>[2x]GAMGRRLGVMGGTFDPIHYGHLVAASEVADLFDLDEVVFVPSGQPWQKGR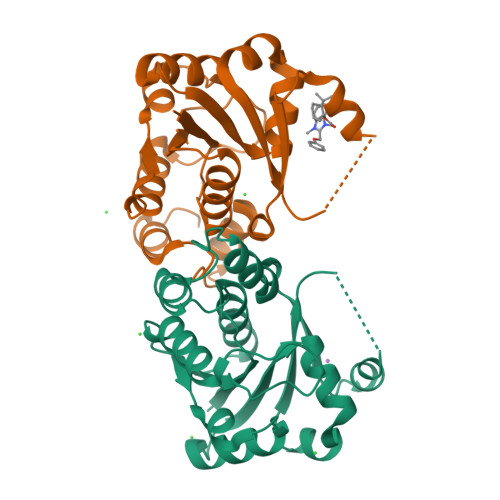QVSAAEHRYLMTVIATASNPRFSVSRVDIDRGGPTYTKDTLADLHALHPDSELYFTTGADALASIMSWQGWEELFELARFVGVSRPGYELRNEHITSLLGQLAKDALTLVEIPALAISSTDCRQRAEQSRPLWYLMPDGVVQYVSKRRLYT> AIGPAASLVVANAPVSPDGFLRDAIVVNGVFPSPLITGKKGDRFQLNVVDTLTNHTMLKSTSIHWHGFFQAGTNWADGPAFVNQCPIASGHSFLYDFHVPDQAGTFWYHSHLSTQYCDGLRGP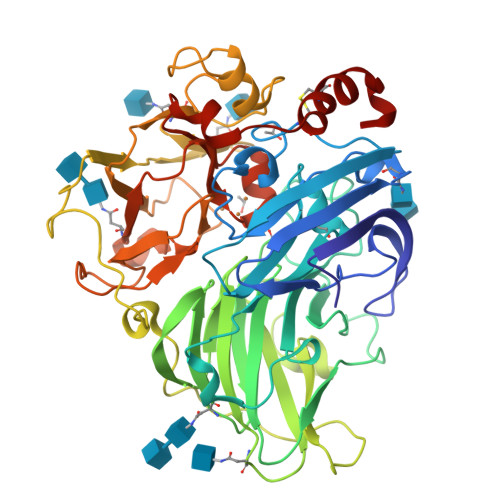FVVYDPKDPHASRYDVDNESTVITLTDWYHTAARLGPRFPLGADATLINGLGRSASTPTAALAVINVQHGKRYRFRLVSISCDPNYTFSIDGHNLTVIEVDGINSQPLLVDSIQIFAAQRYSFVLNANQTVGNYWIRANPNFGTVGFAGGINSAILRYQGAPVAEPTTTQTTSVIPLIETNLHPLARMPVPGSPTPGGVDKALNLAFNFNGTNFFINNASFTPPTVPVLLQILSGAQTAQDLLPAGSVYPLPAHSTIEITLPATALAPGAPHPFHLHGHAFAVVRSAGSTTYNYNDPIFRDVVSTGTPAAGDNVTIRFQTDNPGPWFLHCHIDFHLEAGFAIVFAEDVADVKAANPVPKAWSDLCPIYDGLSEANQ>[3x]PIELLPETPSQTAGPYVHIGLALEAAGNPTRDQEIWNRLAKPDAPGEHILLLGQVYDGNGHLVRDSFLEVWQADANGEYQDAYNLENAFNSFGRTATTFDAGEWTLHTVKPGVVNNAAGVPMAPHINISLFARGINIHLHTRLYFDDEAQANAKCPVLNLIEQPQRRETLIAKRCEVDGKTAYRFDIRIQGEGETVFFDF;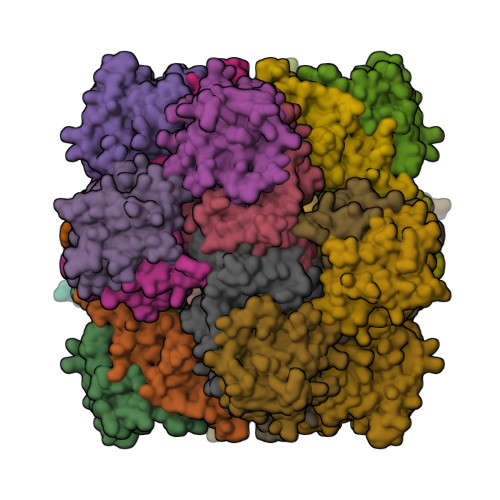>[3x]PAQDNSRFVIRDRNWHPKALTPDYKTSIARSPRQALVSIPQSISETTGPNFSHLGFGAHDHDLLLNFNNGGLPIGERIIVAGRVVDQYGKPVPNTLVEMWQANAGGRYRHKNDRYLAPLDPNFGGVGRCLTDSDGYYSFRTIKPGPAPWRNGPNDWRPAHIYFGISGPSIATKLITQLYFEGDPLIPMCPIVKSIANPEAVQQLIAKLDMNNANPMDCLAYRFDIVLRGQRKTHFENC>[2x]KLANVVILATGGTIAGAGASAANSATYQAAKVGVDKLIAGVPELADLANVRGEQVMQIASESITNDDLLKLGKRVAELADSNDVDGIVITHGTDTLEETAYFLNLVQKTDKPIVVVGSMRPGTAMSADGMLNLYNAVAVASNKDSRGKGVLVTMNDEIQSGRDVSKSINIKTEAFKSAWGPLGMVVEGKSYWFRLPAKRHTVNSEFDIKQISSLPQVDIAYSYGNVTDTAYKALAQ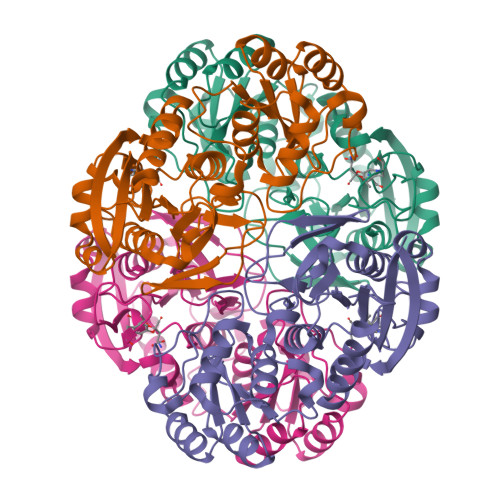NGAKALIHAGTGNGSVSSRVVPALQQLRKNGTQIIRSSHVNQGGFVLRNAEQPDDKNDWVVAHDLNPEKARILAMVAMTKTQDSKELQRIFWEY>MGSSHHHHHHMSVHIEAKQGEIAESILLPGDPLRAKYIAETFLEDVTCYNNVRGMLGFTGTYKGKRVSVQGTGMGVPSISIYVNELIQSYGVKNLIRVGTCGAIQKDVKVRDVIIAMTACTDSNMNRLTFPGFDFAPAANFDLLK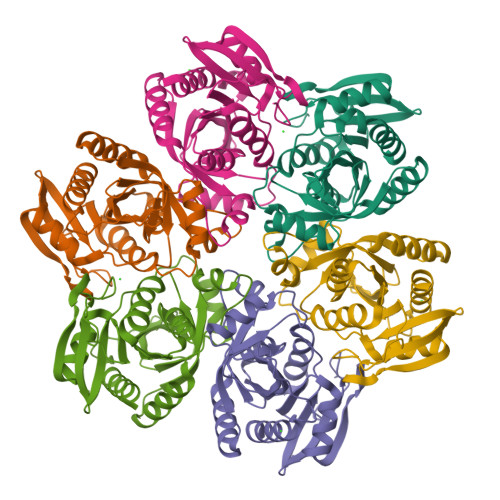KAYDAGTEKGLHVRVGNVLTADVFYRESMDMVKKLGDYGVLAVEMETTALYTLAAKYGVNALSVLTVSDHIFTGEETTSEERQTTFNEMIEIALDAAIQQ[6x]> MNYNNKILVSESGLSQKHLIHGDEELFQHELKTIFARNWLFLTHDSLIPAPGDYVTAKMGIDEVIVSRQNDGSIRAFLNVCRHRGKTLVSVEAGNAKGFVCSYHGWGFGSNGELQSVPFEKDLYGESLNKKCLGLKEVARVESFHGFIYGCFDQEAPPL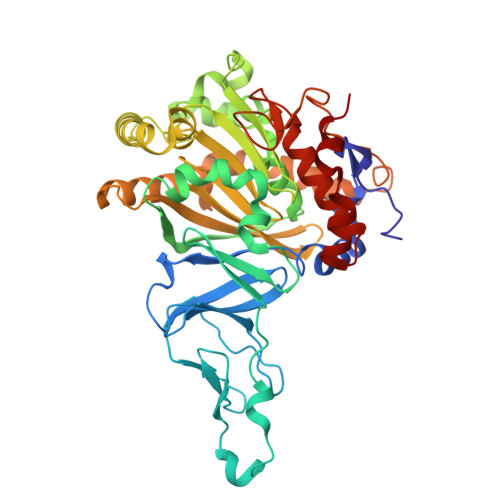MDYLGDAAWYLEPMFKHSGGLELVGPPGKVVIKANWKAPAENFVGDAYHVGWTHASSLRSGESIFSSLAGNAALPPEGAGLQMTSKYGSGMGVLWDGYSGVHSADLVPELMAFGGAKQERLNKEIGDVRARIYRSHLNCTVFPNNSMLTCSGVFKVWNPIDANTTEVWTYAIVEKDMPEDLKRRLADSVQRTFGPAGFWESDDNDNMETASQNGKKYQSRDSDLLSNLGFGEDVYGDAVYPGVVGKSAIGETSYRGFYRAYQAHVSSSNWAEFEHASSTWHTELTKT>SMLTELIASNRRSAAIHAFVDTGLSTHFKDGIYVDISELSRKSGVNYARFSRLCDFLVEMGVLVSNDNKFRLSDECHVFANPESFESFMIKLEICSHYSNAWLMYGKSLFEDDGKSAFEMAHGRPFFEYLDGNKFLKSNFDALMTRVSNLIVEKLLGIYDFNQHNRILDVGGGEGELLVRISEKVKGKHYAVLDRYSELPVSDNIDFINGNFLNSIPSGYDLYILKNVLHNWSDSDSILILENFRKAMDKNSSLLLINMVKEPEFSRSFDILMDVLFLGKE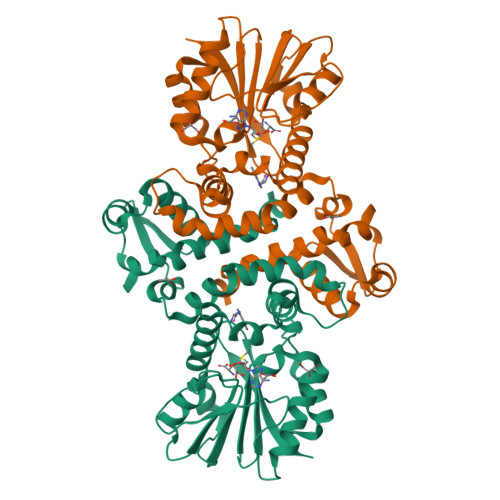RSFTEFEYLANQAGLVVQETKVIDQSYSPYSFIKLQIK[2x]> GSHMAVQIGFLLFPEVQQLDLTGPHDVLASLPDVQVHLIWKEPGPVVASSGLVLQATTSFADCPPLDVICIPGGTGVGALMEDPQALAFIRQQAARARYVTSVCTGSLVLGAAGLLQGKRATTHWAYHELLAPLGAIPVHERVVRDGNLLTGTGITAGIDFALTLAAELFDAATAQRVQLQLEYAPAPPFNAGSPDTAPASVVQQARQRAADSLHKRREITLRAAARLAAG

Here, we address each of these questions in a study of diffuse scattering from crystalline isocyanide hydratase (ICH). We selected the ICH system because it diffracts x-rays to atomic resolution at ambient temperature, has clearly visible diffuse features in ambient temperature x-ray diffraction datasets, and displays large concerted motion of an α-helix that is modulated by the chemical state of the active site nucleophile. Upon formation of the catalytic thioimidate intermediate, this helix becomes more mobile and permits water to enter the active site and complete the reaction.

Engineered mutations at residue 150 (e.g., G150A, G150T) also favor shifted conformations of the helix to varying degrees. As expected based on these structural and space group changes, G150T ICH superimposes onto WT and G150A ICH with a larger Cα RMSD of ∼0.8 Å. In general, the CCLLM values are higher and σ values are lower for the Refmac5 anisotropic ADP models compared to those refined in PHENIX. Considered together, the improved anisotropic ADP CCLLM, the lack of change in CCBragg, the lower values of σ, and the more typical distribution of anisotropies for the Refmac5-refined and rescaled PHENIX anisotropic ADP models show that diffuse scattering data favor anisotropic ADP models that possess more plausible features even when the Bragg models have similar Rfree/Rwork and CCBragg values.> MELPRAFGLLLHPTSLPGPYGVGVLGREARDFLRFLKEAGGRYWQVLPLGPTGYGDSPYQSFSAFAGNPYLIDLRPLAERGYVRLEDPGFPQGRVDYGLLYAWKWPALKEAFRGFKEKASPEEREAFAAFREREAWWLEDYALFMALKGAHGGLPWNRWPLPLRKREEKALREAKSALAEEVAFHAFTQWLFFRQWGALKAEAEALGIRIIGDMPIFVAEDSAEVWAHPEWFHLDEEGRPTVVAGVPPDYFSETGQRWGNPLYRWDVLEREGFSFWIRRLEKALELFHLVRIDHFRGFEAYWEIPASCPTAVEGRWVKAPGEKLFQKIQEVFGEVPVLAEDLGVITPEVEALRDRFGLPGMKVL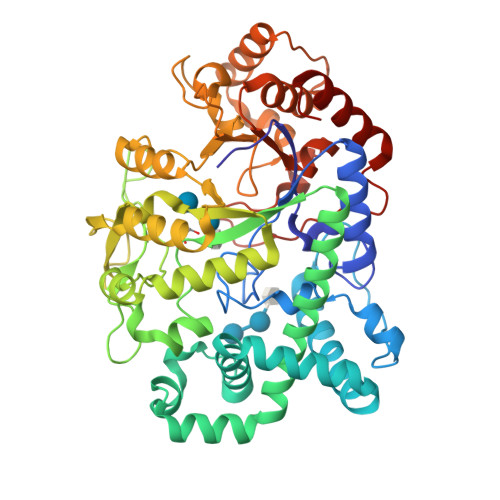QFAFDDGMENPFLPHNYPAHGRVVVYTGTHDNDTTLGWYRTATPHEKAFMARYLADWGITFREEEEVPWALMHLGMKSVARLAVYPVQDVLALGSEARMNYPGRPSGNWAWRLLPGELSPEHGARLRAMAEATERL>[3x]MRMIVGHGIDIEELASIESAVTR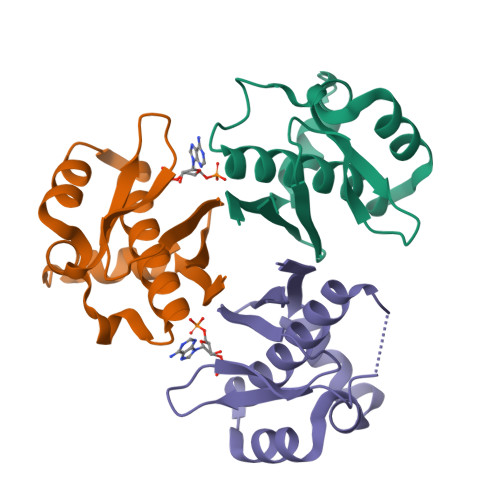HEGFAKRVLTALEMERFTSLKGRRQIEYLAGRWSAKEAFSKAMGTGISKLGFQDLEVLNNERGAPYFSQAPFSGKIWLSISHTDQFVTASVILEENHES>[2x]MAHHHHHHMSTSLSYRDAGVGIDAGDQLVEKIKPFAKRTMRPEVLGDLGGFGALVEIGKKYQNPVLVSGTDGVGTKLKLAFDWDKHDTVGIDLVAMSVNDILVQGAEPLFFLDYFA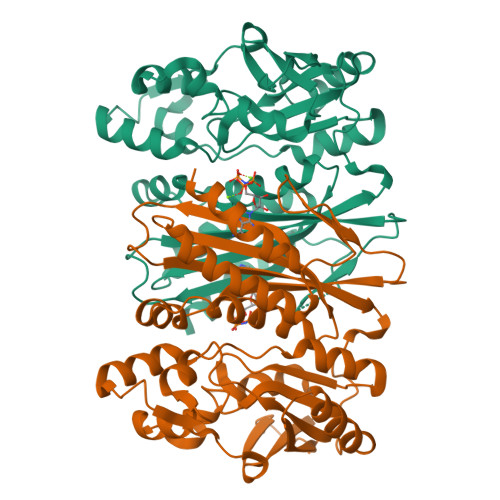CGKLDVPRATDVIKGIAQGCEESGCALIGGETAEMPGMYPVGEYDLAGFAVGVVEKENVITGLSVGAGDMVLGLASNGAHSNGYSLIRKIIERDNPDLDAEFDNGKTLREAVIAPTRLYVKPILAALEKFTIKGMAHITGGGITENVPRVLPKNTVAQIDAESWELPKLFQWLQKAGNVETQEMYRTFNCGIGMVVIVAAEDADAVRSFLSGQGETVYRLGCIRERQGNEHQTQVA2-((3',5'-DIMETHYL-4'-HYDROXYPHENYL)AZO)BENZOIC ACID 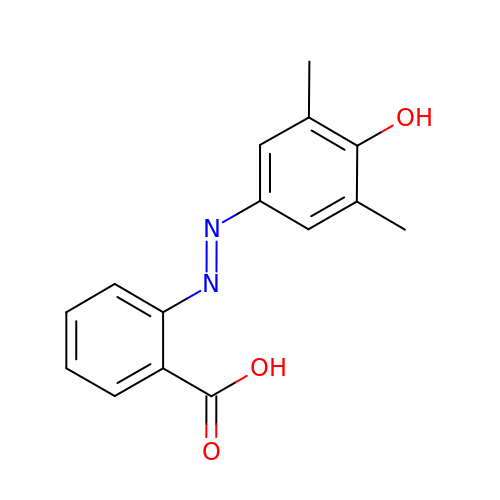| C15 H14 N2 O3 | ZMDQWZFZPGJFPM-WUKNDPDISA-N CC chemokine ligands (CCL) comprise 8-14 kDa chemotactic cytokines (chemokines) involved in diverse immune functions. Extensive structural analyses reveal that most chemokines share a common core structure: an N-terminal extension followed by a 310 helical turn, an anti-parallel three-stranded β-sheet, and an α-helix. CC chemokines also readily dimerize, primarily through the formation of an anti-parallel β-sheet at their N-termini. Certain chemokines, e.g. CCL3, CCL4, and CCL5 form polydisperse, high MW reversible polymers in excess of 600 kDa without the assistance of GAG.

Mutation of Proline 8 to alanine (P8A) profoundly reduces the polymerization of CCL3 and CCL4. CCL3 P8A crystallized in space group P6222. There are five CCL3 molecules in each asymmetric unit. CCL3 P8A still arranges as a polymer structure similar to wild type CCL3; each dimer rotates 36° to bind to the adjacent dimer such that a decamer completes a 180° turn. However, the N-termini of CCL3 P8A exhibit substantial heterogeneity, indicating that these N termini are more disordered than wild type CCL3 and can adopt multiple conformations. One such conformation results in the loss of a hydrogen bond between D6 and S33 in CCL3 P8A. This disrupts a key contact between CCL3 dimers. The loss of contact between CCL3 dimers and the conformational disorder of CCL3 N-termini likely contribute to the decreased stability of the CCL3 polymer, leading to depolymerization. In the CCL3 structure, however, the P8A substitution disrupts crucial contacts between CCL3 dimers to reduce the formation of CCL3 polymers without affecting the dimer formation of CCL3.

>ASLAADTATACCFSYTSRQIPQNFIADYFETSSQCSKPGVIFLTKRSRQVCADPSEEWVQKYVSDLELS[5x]>SMDLNINDDPNYPMNDQVTADLIFPSISASIASAVGGEIYNYAGFFAQYYEQKPESNQYNTLCEYTFTESSQQMDYSYRILFAGALEDAKQVLEKTTNPADRFATTILRAYAFQIMVDNTSDSPYSEALQGNANATPKWDTGETVYKGILGEIDAAEAALDGSGMDVPDLIFNKNIAQWKGFANALRLRMYLRFIDANIDAASYTEKVKTLVQNNEFFTGDVKLDCFLDETDKRNPWYNTNAVGLTGNHCAAYPLVSYLSSTGDPRIAYGISKTDADGKYVGQLPGGKTHMQSILGTDNWKNKNVSAIDYSIGATKPVYFFTQAELQFLIAEVYARFHNDDANAKSAYEAGVTADFAVRGFAGQENTILEGACAWSAASTQADKLNLIYMQKWVSLFYMDHMEAWSEIRRTDCPKLSSYSAAQIQASESVYTPGELVAPWTNG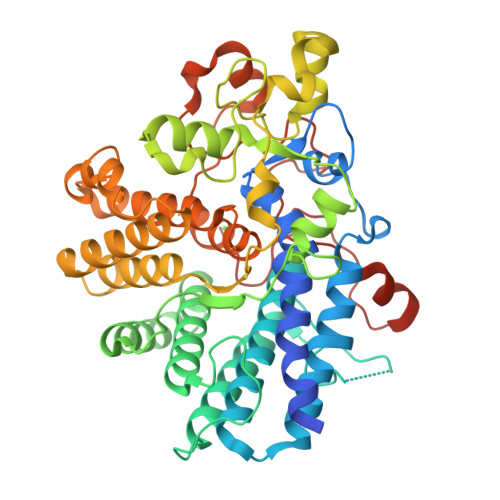LEAGGLMKRMTYPLSARQQNVNTPAGVPGSTPVWWDIK[2x]> GUGTAX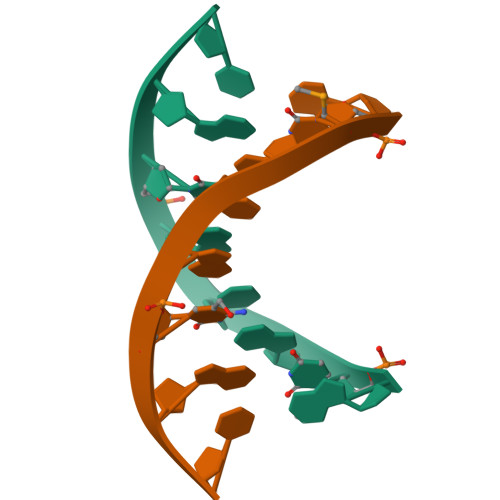AC> MDFQHRPGGKTGSGGVASSSESNRDRRERLRQLALETIDINKDPYFMKNHLGSYECKLCLTLHNNEGSYLAHTQGKKHQTNLARRAAKEAKEAPAQPAPEKVKVEVKKFVKIGRPGYKVTKQRDSEMGQQSLLFQIDYPEIAEGIMPRHRFMSAYEQRIEPPDRRWQYLLMAAEPYETIAFKVPSREIDKAEGKFWTHWNRETKQFFLQFHFKMEKPPAPPSLPAGPPGVKRPPPPLMNGLPPRPPLPESLPPPPPGGLPLPPMPPTGPAPSGPPGPPQLPPPAPGVHPPAPVVHPPASGVHPPAPGVHPPAPGVHPPAPGVHPPTSGVHPPAPGVHPPAPGVHPPAPGVHPPAPGVHPPAPGVHPPPSAGVHPQAPGVHPAAPAVHPQAPGVHPPAPGMHPQAPGVHPQPPGVHPSAPGVHPQPPGVHPSNPGVHPPTPMPPMLRPPLPSEGPGNIPPPPPTN;> METILEQQRRYHEEKERLMDVMAKEMLTKKSTLRDQINSDHRTRAMQDRYMEVSGNLRDLYDDKDGLRKEELNAISGPNEFAEFYNRLKQIKEFHRKHPNEICVPMSVEFEELLKARENPSEEAQNLVEFTDEEGYGRYLDLHDCYLKYINLKASEKLDYITYLSIFDQLFDIPKERKNAEYKRYLEMLLEYLQDYTDRVKPLQDQNELFGKIQAEFEKKWENGTFPGWPKETSSALTHAGAHLDLSAFSSWEELASLGLDRLKSALLALGLKCGGTLEERAQRLFSTKGKSLESLDTSLFAKNPKSKGTKRDTERNKDIAFLEAQIYEYVEILGEQRHLTHENVQRKQARTGEEREEEEEEQISESESEDEENEIIYNPKNLPLGWDGKPIPYWLYKLHGLNINYNCEICGNYTYRGPKAFQRHFAEWRHAHGMRCL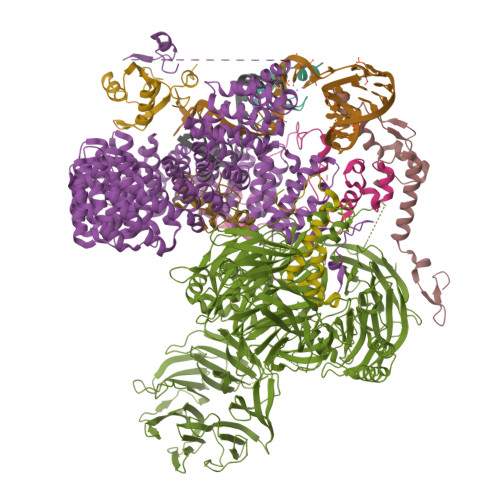GIPNTAHFANVTQIEDAVSLWAKLKLQKASERWQPDTEEEYEDSSGNVVNKKTYEDLKRQGLL;> MAKIAKTHEDIEAQIREIQGKKAALDEAQGVGLDSTGYYDQEIYGGSDSRFAGYVTSIAATELEDDDDDYSSSTSLLGQKKPGYHAPVALLNDIPQSTEQYDPFAEHRPPKIADREDEYKKHRRTMIISPERLDPFADGGKTPDPKMNARTYMDVMREQHLTKEEREIRQQLAEKAKAGELKVVNGAAASQPPSKRKRRWDQTADQTPGATPKKLSSWDQAETPGHTPSLRWDETPGRAKGSETPGATPGSKIWDPTPSHTPAGAATPGRGDTPGHATPGHGGATSSARKNRWDETPKTERDTPGHGSGWAETPRTDRGGDSIGETPTPGASKRKSRWDETPASQMGGSTPVLTPGKTPIGTPAMNMATPTPGHIMSMTPEQLQAWRWEREIDERNRPLSDEELDAMFPEGYKVLPPPAGYVPIRTPARKLTATPTPLGGMTGFHMQTEDRTMKSVNDQPSGNLPFLKPDDIQYFDKLLVDVDESTLSPEEQKERKIMKLLLKIKNGTPPMRKAALRQITDKAREFGAGPLFNQILPLLMSPTLEDQERHLLVKVIDRILYKLDDLVRPYVHKILVVIEPLLIDEDYYARVEGREIISNLAKAAGLATMISTMRPDIDNMDEYVRNTTARAFAVVASALGIPSLLPFLKAVCKSKKSWQARHTGIKIVQQIAILMGCAILPHLRSLVEIIEHGLVDEQQKVRTISALAIAALAEAATPYGIESFDSVLKPLWKGIRQHRGKGLAAFLKAIGYLIPLMDAEYANYYTREVMLILIREFQSPDEEMKKIVLKVVKQCCGTDGVEANYIKTEILPPFFKHFWQHRMALDRRNYRQLVDTTVELANKVGAAEIISRIVDDLKDEAEQYRKMVMETIEKIMGNLGAADIDHKLEEQLIDGILYAFQEQTTEDSVMLNGFGTVVNALGKRVKPYLPQICGTVLWRLNNKSAKVRQQAADLISRTAVVMKTCQEEKLMGHLGVVLYEYLGEEYPEVLGSILGALKAIVNVIGMHKMTPPIKDLLPRLTPILKNRHEKVQENCIDLVGRIADRGAEYVSAREWMRICFELLELLKAHKKAIRRATVNTFGYIAKAIGPHDVLATLLNNLKVQERQNRVCTTVAIAIVAETCSPFTVLPALMNEYRVPELNVQNGVLKSLSFLFEYIGEMGKDYIYAVTPLLEDALMDRDLVHRQTASAVVQHMSLGVYGFGCEDSLNHLLNYVWPNVFETSPHVIQAVMGALEGLRVAIGPCRMLQYCLQGLFHPARKVRDVYWKIYNSIYIGSQDALIAHYPRIYNDDKNTYIRYELDYIL;> MATEHPEPPKAELQLPPPPPPGHYGAWAAQELQAKLAEIGAPIQGNREELVERLQSYTRQTGIVLNRPVLRGEDGDKAAPPPMSAQLPGIPMPPPPLGLPPLQPPPPPPPPPPGLGLGFPMAHPPNLGPPPPLRVGEPVALSEEERLKLAQQQAALLMQQEERAKQQGDHSLKEHELLEQQKRAAVLLEQERQQEIAKMGTPVPRPPQDMGQIGVRTPLGPRVAAPVGPVGPTPTVLPMGAPVPRPRGPPPPPGDENREMDDPSVGPKIPQALEKILQLKESRQEEMNSQQEEEEMETDARSSLGQSASETEEDTVSVSKKEKNRKRRNRKKKKKPQRVRGVSSESSGDREKDSTRSRGSDSPAADVEIEYVTEEPEIYEPNFIFFKRIFEAFKLTDDVKKEKEKEPEKLDKLENSAAPKKKGFEEEHKDSDDDSSDDEQEKKPEAPKLSKKKLRRMNRFTVAELKQLVARPDVVEMHDVTAQDPKLLVHLKATRNSVPVPRHWCFKRKYLQGKRGIEKPPFELPDFIKRTGIQEMREALQEKEEQKTMKSKMREKVRPKMGKIDIDYQKLHDAFFKWQTKPKLTIHGDLYYEGKEFETRLKEKKPGDLSDELRISLGMPVGPNAHKVPPPWLIAMQRYGPPPSYPNLKIPGLNSPIPESCSFGYHAGGWGKPPVDETGKPLYGDVFGTNAAEFQTKTEEEEIDRTPWGELEPSDEESSEEEEEEESDEDKPDETGFITPADSGLITPGGFSSVPAGMETPELIELRKKKIEEAMDGSETPQLFTVLPEKRTATVGGAMMGSTHIYDMSTVMSRKGPAPELQGVEVALAPEELELDPMAMTQKYEEHVREQQAQVEKEDFSDMVAEHAAKQKQKKRKAQPQDSRGGSKKYKEFKF;> MFLYNLTLQRATGISFAIHGNFSGTKQQEIVVSRGKILELLRPDPNTGKVHTLLTVEVFGVIRSLMAFRLTGGTKDYIVVGSDSGRIVILEYQPSKNMFEKIHQETFGKSGCRRIVPGQFLAVDPKGRAVMISAIEKQKLVYILNRDAAARLTISSPLEAHKANTLVYHVVGVDVGFENPMFACLEMDYEEADNDPTGEAAANTQQTLTFYELDLGLNHVVRKYSEPLEEHGNFLITVPGGSDGPSGVLICSENYITYKNFGDQPDIRCPIPRRRNDLDDPERGMIFVCSATHKTKSMFFFLAQTEQGDIFKITLETDEDMVTEIRLKYFDTVPVAAAMCVLKTGFLFVASEFGNHYLYQIAHLGDDDEEPEFSSAMPLEEGDTFFFQPRPLKNLVLVDELDSLSPILFCQIADLANEDTPQLYVACGRGPRSSLRVLRHGLEVSEMAVSELPGNPNAVWTVRRHIEDEFDAYIIVSFVNATLVLSIGETVEEVTDSGFLGTTPTLSCSLLGDDALVQVYPDGIRHIRADKRVNEWKTPGKKTIVKCAVNQRQVVIALTGGELVYFEMDPSGQLNEYTERKEMSADVVCMSLANVPPGEQRSRFLAVGLVDNTVRIISLDPSDCLQPLSMQALPAQPESLCIVEMGGTEKQDELGERGSIGFLYLNIGLQNGVLLRTVLDPVTGDLSDTRTRYLGSRPVKLFRVRMQGQEAVLAMSSRSWLSYSYQSRFHLTPLSYETLEFASGFASEQCPEGIVAISTNTLRILALEKLGAVFNQVAFPLQYTPRKFVIHPESNNLIIIETDHNAYTEATKAQRKQQMAEEMVEAAGEDERELAAEMAAAFLNENLPESIFGAPKAGNGQWASVIRVMNPIQGNTLDLVQLEQNEAAFSVAVCRFSNTGEDWYVLVGVAKDLILNPRSVAGGFVYTYKLVNNGEKLEFLHKTPVEEVPAAIAPFQGRVLIGVGKLLRVYDLGKKKLLRKCENKHIANYISGIQTIGHRVIVSDVQESFIWVRYKRNENQLIIFADDTYPRWVTTASLLDYDTVAGADKFGNICVVRLPPNTNDEVDEDPTGNKALWDRGLLNGASQKAEVIMNYHVGETVLSLQKTTLIPGGSESLVYTTLSGGIGILVPFTSHEDHDFFQHVEMHLRSEHPPLCGRDHLSFRSYYFPVKNVIDGDLCEQFNSMEPNKQKNVSEELDRTPPEVSKKLEDIRTRYAF;> MTDRYTIHSQLEHLQSKYIGTGHADTTKWEWLVNQHRDSYCSYMGHFDLLNYFAIAENESKARVRFNLMEKMLQPCGPPADKPEEN;> MAMQAAKRANIRLPPEVNRILYIRNLPYKITAEEMYDIFGKYGPIRQIRVGNTPETRGTAYVVYEDIFDAKNACDHLSGFNVCNRYLVVLYYNANRAFQKMDTKKKEEQLKLLKEKYGINTDPPK;> MAKHHPDLIFCRKQAGVAIGRLCEKCDGKCVICDSYVRPCTLVRICDECNYGSYQGRCVICGGPGVSDAYYCKECTIQEKDRDGCPKIVNLGSSKTDLFYERKKYGFKKR>GSFSKEESREFMAIFPDIVRDLTDAGRHTDIPEVTKRFAKVLQYNVPTGKKTRGLSTVIAYKMLEKPENLTPENVRLAGILGWCVELLQASLLIMDDLMDRSETRRGQPCWYRQENVGFLAINDCLHVESSLYSVLRKYFSHLPCYVPIIELFHDVNFKTNMGQSLDALCMKDGRPILSQFTMKRYSSIVKYKTSYYTFQLPVSLGMYLADMYDPEQHRQAKTILMEIGEFFQIQDDFLDAFGDSQVTGKVGTDIKEGKCSWLAVVALQRSNPAQRQIMEEHYGRPEPESTQIIKNLYIELGLPATFAVYEEESFNIIRTHIHQISKGLPHDLFFKAMKKIYKRDA[2x]

Here we characterize a metal-dependent, bifunctional isoprenyl diphosphate synthase from the leaf beetle Phaedon cochleariae by structural and functional analyses. Isoprenyl diphosphate synthase in P. cochleariae (PcIDS1, EC 2.5.1.1) produces FPP in the presence of Mg2+, but preferably forms GPP when exposed to the heavy metal ions (HMIs) Co2+ or Mn2+. Inter- and intramolecular cooperative effects in the homodimer strongly depend on the provided metal ions and regulate the biosynthetic flux of terpene precursors to either biological defence or physiological development. Strikingly, a unique chain length determination domain adapts to form geranyl or farnesyl pyrophosphate by altering enzyme symmetry and ligand affinity between both subunits.

V286 and I420 form the bottom of this specificity pocket and act as a molecular ruler, whereas F282 and F315 engage in π-stacking with both allyl groups. However, the human FPPAllo does not interact with the substrate loop and protrudes into a 4-Å-deeper cavity by inverting the prenyl moiety. This orientation is stabilized by L344, whereas the corresponding I420 in PcIDS1 tailors the allosteric binding channel to GPP.> MNMLALTIILPLIGFVLLAFSRGRWSENVSAIVGVGSVGLAALVTAFIGVDFFANGEQTYSQPLWTWMSVGDFNIGFNLVLDGLSLTMLSVVTGVGFLIHMYASWYMRGEEGYSRFFAYTNLFIASMVVLVLADNLLLMYLGWEGVGLCSYLLIGFYYTDPKNGAAAMKAFVVTRVGDVFLAFALFILYNELGTLNFR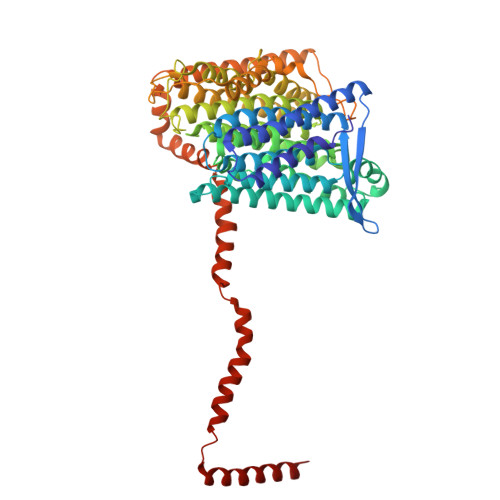EMVELAPAHFADGNNMLMWATLMLLGGAVGKSAQLPLQTWLADAMAGPTPVSALIHAATMVTAGVYLIARTHGLFLMTPEVLHLVGIVGAVTLLLAGFAALVQTDIKRVLAYSTMSQIGYMFLALGVQAWDAAIFHLMTHAFFKALLFLASGSVILACHHEQNIFKMGGLRKSIPLVYLCFLVGGAALSALPLVTAGFFSKDEILAGAMANGHINLMVAGLVGAFMTSLYTFRMIFIVFHGKEQIHAHAVKGVTHSLPLIVLLILSTFVGALIVPPLQGVLPQTTELAHGSMLTLEITSGVVAVVGILLAAWLWLGKRTLVTSIANSAPGRLLSTWWYNAWGFDWLYDKVFVKPFLGIAWLLKRDPLNSMMNIPAVLSRFAGKGLLLSENGYLRWYVASMSIGAVVVLALLMVLR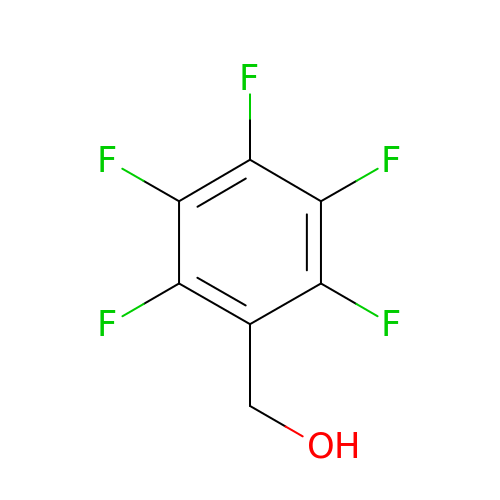2,3,4,5,6-PENTAFLUOROBENZYL ALCOHOL | C7 H3 F5 O | PGJYYCIOYBZTPU-UHFFFAOYSA-N> GGUUGCCGAA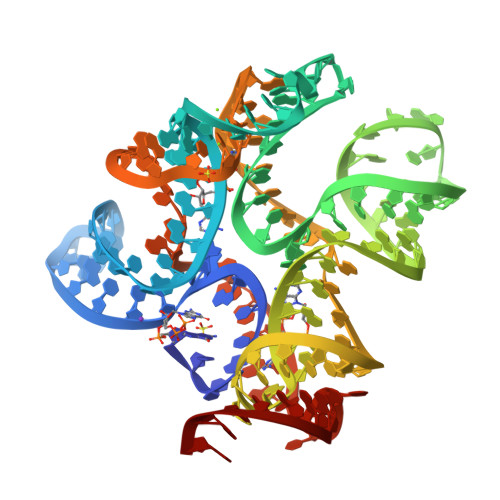UCCGAUGCUCGGUACGGAGGAACCGCUUUUUGGGGUUAAUCUGCAGUGAAGCUGCAGUAGGGAUACCUUCUGUCCCGCACCCGACAGCUAACUCCGGAGGCAAUAAAGGAAGGAG>[2x]DLEERFERLYEKAKKLAEERGDERARRMIELLRQLFETVGDPRILELLELLL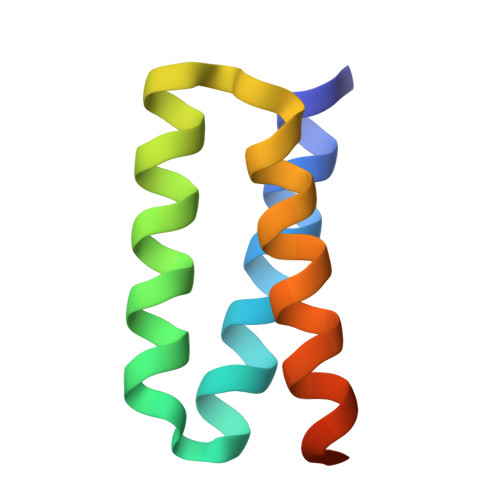QLLEGLEHHHHHH>[3x]SVEPLSVNGNKIYAGEKAKSFAGNSLFWSNNGWGGEKFYTADTVASLKKDWKSSIVRAAMGVQESGGYLQDPAGNKAKVERVVDAAIANDMYA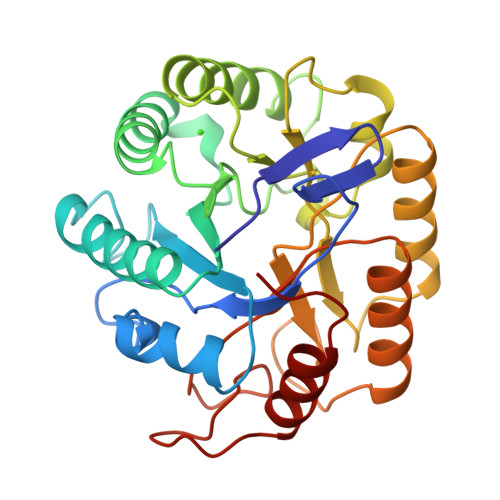IIGWHSHSAENNRSEAIRFFQEMARKYGNKPNVIYEIYNEPLQVSWSNTIKPYAEAVISAIRAIDPDNLIIVGTPSWSQNVDEASRDPINAKNIAYTLHFYAGTHGESLRNKARQALNNGIALFVTEWGTVNADGNGGVNQTETDAWVTFMRDNNISNANWALNDKNEGASTYYPDSKNLTESGKKVKSIIQSWPYKA> MKHHHHHHSAGLEVLFQGPGTGSEFELMMFGKKKNNGGSSTARYSAGNKYNTLSNNYALSAQQLLNASKIDDIDSMMGFERYVPPQYNGRFDAKDIDQIPGRVGWLTNMHATLVSQETLSSGSNGGGNSNDGERVTTNQGISGVDFYFLDEEGGSFKSTVVYDPYFFIACNDESRVNDVEELVKKYLESCLKSLQIIRKEDLTMDNHLLGLQKTLIKLSFVNSNQLFEARKLLRPILQDNANNNVQRNIYNVAANGSEKVDAKHLIEDIREYDVPYHVRVSIDKDIRVGKWYKVTQQGFIEDTRKIAFADPVVMAFAIATTKPPLKFPDSAVDQIMMISYMIDGEGFLITNREIISEDIEDFEYTPKPEYPGFFTIFNENDEVALLQRFFEHIRDVRPTVISTFNGDFFDWPFIHNRSKIHGLDMFDEIGFAPDAEGEYKSSYCSHMDCFRWVKRDSYLPQGSQGLKAVTQSKLGYNPIELDPELMTPYAFEKPQHLSEYSVSDAVATYYLYMKYVHPFIFSLCTIIPLNPDETLRKGTGTLCEMLLMVQAYQHNILLPNKHTDPIERFYDGHLLESETYVGGHVESLEAGVFRSDLKNEFKIDPSAIDELLQELPEALKFSVEVENKSSVDKVTNFEEIKNQITQKLLELKENNIRNELPLIYHVDVASMYPNIMTTNRLQPDSIKAERDCASCDFNRPGKTCARKLKWAWRGEFFPSKMDEYNMIKRALQNETFPNKNKFSKKKVLTFDELSYADQVIHIKKRLTEYSRKVYHRVKVSEIVEREAIVCQRENPFYVDTVKSFRDRRYEFKGLAKTWKGNLSKIDPSDKHARDEAKKMIVLYDSLQLAHKVILNSFYGYVMRKGSRWYSMEMAGITCLTGATIIQMARALVERVGRPLELDTDGIWCILPKSFPETYFFTLENGKKLYLSYPCSMLNYRVHQKFTNHQYQELKDPLNYIYETHSENTIFFEVDGPYKAMILPSSKEEGKGIKKRYAVFNEDGSLAELKGFELKRRGELQLIKNFQSDIFKVFLEGDTLEGCYSAVASVCNRWLDVLDSHGLMLEDEDLVSLICENRSMSKTLKEYEGQKSTSITTARRLGDFLGEDMVKDKGLQCKYIISSKPFNAPVTERAIPVAIFSADIPIKRSFLRRWTLDPSLEDLDIRTIIDWGYYRERLGSAIQKIITIPAALQGVSNPVPRVEHPDWLKRKIATKEDKFK;> MSINLHSAPEYDPSYKLIQLTPELLDIIQDPVQNHQLRFKSLDKDKSEVVLCSHDKTWVLKQRKHSNTVLLMREFVPEQPITFDETLLFGLSKPYMDVVGFAKTESEFETRETHGELNLNSVPIYNGELDFSDKIMKRSSTKVIGTLEELLENSPCSALEGISKWHKIGGSVKDGVLCILSQDFLFKALHVLLMSAMAESLDLQHLNVEDTHHAVGKDIEDEFNPYTREIIETVLNKFAVQEQEAENNTWRLRIPFIAQWYGIQALRKYVSGISMPIDEFLIKWKSLFPPFFPCDIDIDMLRGYHFKPTDKTVQYIAKSTLPMDPKERFKVLFRLQSQWDLEDIKPLIEELNSRGMKIDSFIMKYARRKRLGKKTVVTSR;> MPSVDIDASQWQKLTQSREKQTTVITPLGMMMLEIQGELELPKDFASLARRDSPNEGRFSEQDGETLIRFGSLQIDGERATLFVGKKQRLLGKVTKLDVPMGIMHFNSKDNKVELVDVMKYKVIFKDRPLPIM;> GAMGNQTVKIWVKYNEGFSNAVRKNVTWNNLWE

Ctf18-RFC belongs to the RFC family of AAA+ ATPase clamp loaders, which are involved in the loading and unloading of clamps onto dsDNA. Compared to other clamp loaders, Ctf18-RFC contains two additional subunits, Ctf8 and Dcc1, which bind to the C-terminus of Ctf18 to form the Ctf18-1-8 module. Mutations in Ctf18 that disrupt formation of this Ctf18-1-8 module result in similar but not identical phenotypes as entire deletions of Ctf18 (29,30), suggesting that this module is critical for at least some of the specialized functions of Ctf18-RFC. It has been shown that the Ctf18-1-8 module binds the N-terminal catalytic domain of Pol2 (30,31), the largest subunit of the leading strand Pol ϵ, and that this interaction increases the clamp loader activity of Ctf18-RFC.

We next investigated the mechanism by which the large interaction interface could adapt to the conformational changes of Pol2CAT that would occur during DNA synthesis. As we were unable to solve a DNA-bound structure of the complex, we instead obtained clear insight into how the interaction behaves in different Pol2CAT conformations by refining a second lower-resolution (5.8 Å) cryo-EM class (Class 2). In Class 2, while the majority of Pol2CAT remains in the same position, Pol2THUMB has undergone a small movement. To maintain simultaneous interaction at all three patches despite this movement, the entirety of Ctf18-1-8 has rotated. While the central highly specific interface is unchanged, the Dcc1WH3–Pol2EXO interaction is completely altered. This plasticity can be explained by the non-specific and electrostatic nature of this interface. We show this is achieved through an unusual protein–protein mechanism that utilizes flexible electrostatic interfaces to enable high binding plasticity.> GPLGSMALVAPEAPSEQARRVFQTYDPEDNGFIPDSLLEDVMKA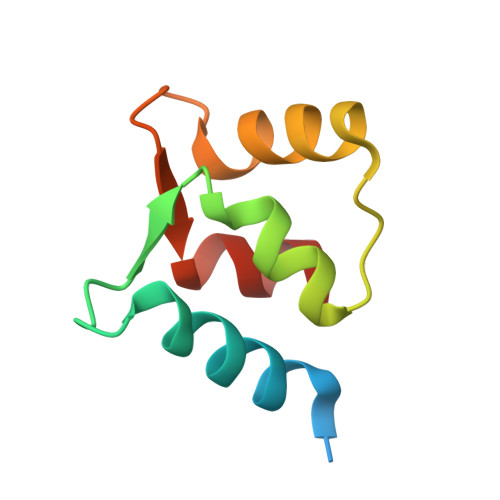LDLVSDPEYINLMKNKLDPEGLGIILLGPFLQEFFP> GAMGEPPLATRATAPPGVLKIFGAGLASGANYKSVLATARSTARELVAEALERYGLAGSPGGGPGESSCVDAFALCDALGRPAAAGVGSGEWRAEHLRVLGDSERPLLVQELWRARPGWARRFELR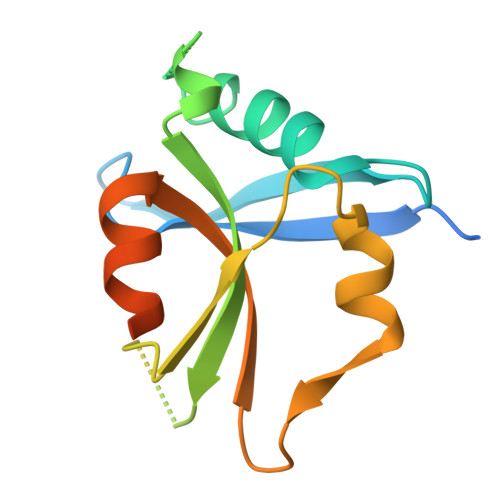GREEARRLEQEAFGAADSEGTGAPSWRPQK> MPVFHTRTIESILEPVAQQISHLVIMHEEGEVDGKAIPDLTAPVAAVQAAVSNLVRVGKETVQTTEDQILKRDMPPAFIKVENACTKLVQAAQMLQSDPYSVPARDYLIDGS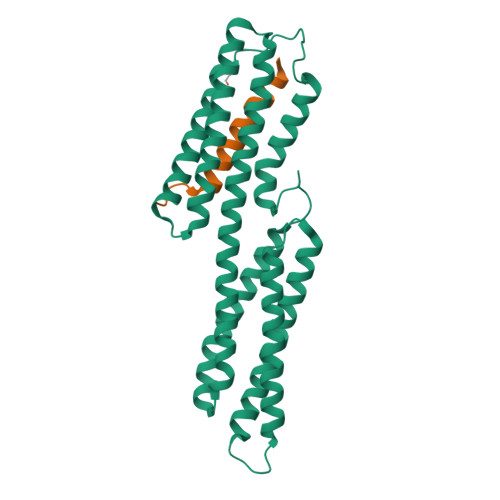RGILSGTSDLLLTFDEAEVRKIIRVCKGILEYLTVAEVVETMEDLVTYTKNLGPGMTKMAKMIDERQQELTHQEHRVMLVNSMNTVKELLPVLISAMKIFVTTKNSKNQGIEEALKNRNFTVEKMSAEINEIIRVLQLTSWDE;> GSHMNLLNAATALSGSMQYLLNYVNAG>[2x]MGSSHHHHHHSSGLVPRGSPQCHFDIEINREPVGRIMFQLFSDICPKTCKNFLCLCSGEKGLGKTTGKKLCYKGSTFHRVVKNFMIQGGDFSEGNGKGGES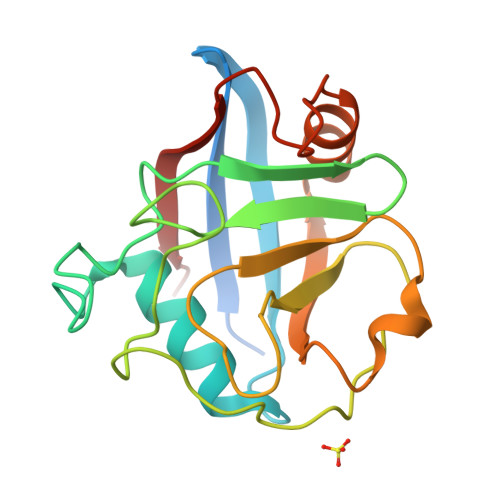IYGGYFKDENFILKHDRAFLLSMANRGKHTNGSQFFITTKPAPHLDGVHVVFGLVISGFEVIEQIENLKTDAASRPYADVRVIDCGVLATK>[2x]MGSITENTSWNKEFSAEAVNGVFVLCKSSSKSCATNDLARASKEYLPASTFKIPNAII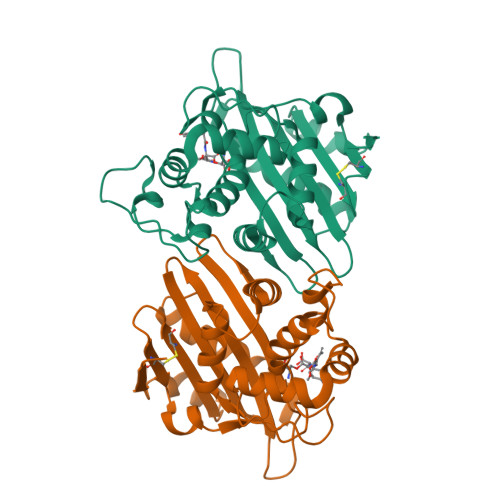GLETGVIKNEHQVFKWDGKPRAMKQWERDLTLRGAIQVSAVPVFQQIAREVGEVRMQKYLKKFSYGNQNISGGIDKFWLEGQLRISAVNQVEFLESLYLNKLSASKENQLIVKEALVTEAAPEYLVHSKTGFSGVGTESNPGVAWWVGWVEKETEVYFFAFNMDIDNESKLPLRKSIPTKIMESEGIIGG>[4x]GGCUAGCUGGAGGGGCGCCAGU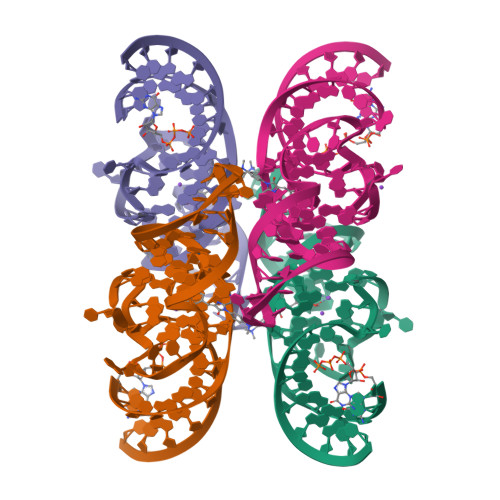UCGCUGGUGGUUGGGUGCGGUCGGCUAGCC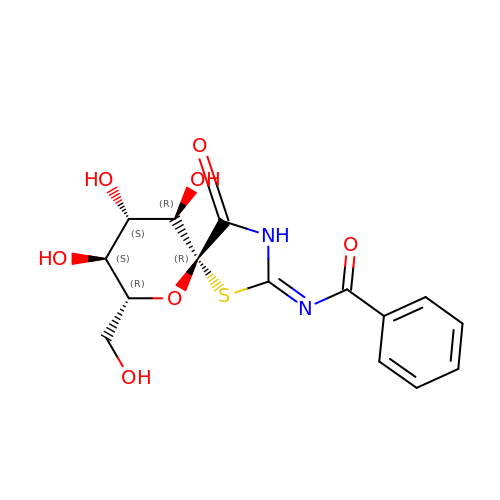N-[(2Z,5R,7R,8S,9S,10R)-8,9,10-trihydroxy-7-(hydroxymethyl)-4-oxo-6-oxa-1-thia-3-azaspiro[4.5]dec-2-ylidene]benzamide | C15 H16 N2 O7 S | FROKMWINLHSJAI-XKJBLICVSA-N> PRK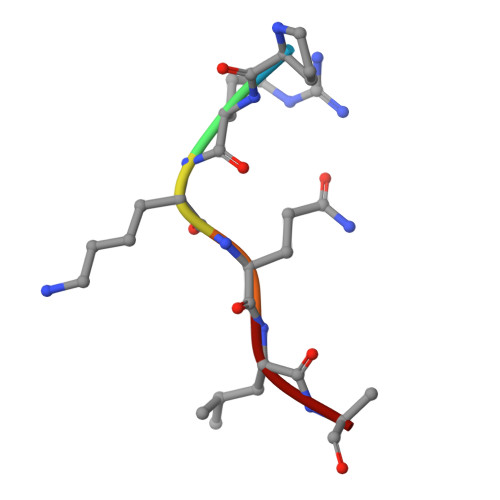QLA>[2x]SAKLECPQDWLSHRDKCFRVSQVSNTWEEGLVDCDGKGATLMLIQDQEELRFLLDS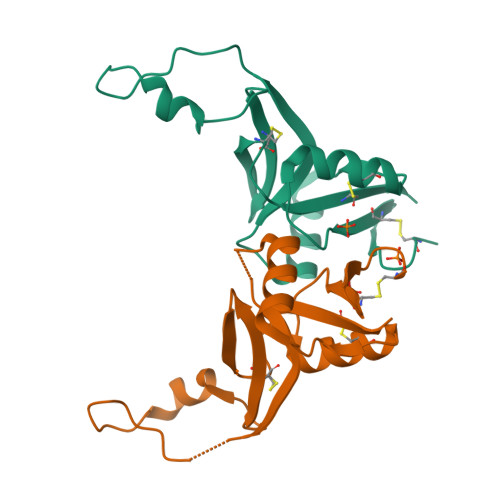IKEKYNSFWIGLRYTLPDMNWKWINGSTLNSDVLKITGDTENDSCAAISGDKVTFESCNSDNRWICQKELYHETLSNYVGYGH In such microorganisms, the majority of small molecules are taken up by members of the OprD outer membrane protein family. Here we show that OprD channels require a carboxyl group in the substrate for efficient transport, and based on this we have renamed the family Occ, for outer membrane carboxylate channels. As expected from pairwise sequence identities that range from 35%–50%, the Occ proteins share a similar architecture, with a slightly off-center constriction formed by the inward-folded extracellular loops L3 and L7 and residues in the barrel wall. The transport data demonstrate that Occ channels have a pronounced preference for substrates with a carboxyl group, due to the universal presence of a basic ladder on one side of the barrel wall.

In addition to these new structures, we obtained much higher resolution data and more complete structures for OccD1 (formerly OprD; 2.15 Å versus 2.9 Å previously) and OccK1 (formerly OpdK; 1.65 Å versus 2.8 Å previously). As a comparison, the OccK1 pore is slightly larger in diameter than that of E. coli LamB, which is a channel specific for sugars. For OccK channels, conductance values are on average somewhat larger than those of OccD subfamily members, ranging from ∼50 pS for OccK4 to ∼300 pS for OccK1, OccK5, and OccK7. Vanillate, while being transported by OccK1, is clearly not the preferred substrate for this channel since relatively high substrate concentrations (10 µM) and long uptake times had to be used to obtain relatively low specific activities. This result is consistent with previous single-channel experiments, where the affinity of vanillate for OccK1 was found to be quite low (∼2 mM). Notably, while the current OccK1 structure contains two vanillate molecules, they are not bound at positions relevant for transport, confirming that vanillate is not a good substrate for OccK1. An interesting finding is the efficient lowering of OccK1-mediated benzoate transport by octanoate and caproate, suggesting that OccK1, but not OccD1 and OccK2, can serve as an uptake channel for medium-chain and possibly short-chain fatty acids. OccK1 is the least specific channel, also allowing the efficient passage of certain linear compounds such as medium-chain fatty acids. As judged by the inhibition of transport, OccK1 interacts with carbenicillin and cefoxitin. Intriguingly, OccK1-mediated transport is also affected by tetracycline, which is a non-β-lactam polyketide compound that does not have a carboxyl group.

>[2x]AEGGFLEDAKTDLVLRNYYFNRDFRDHDAGKSLVDEWAQGFILKFSSGYTPGTVGVGLDAIGLFGVKLNSGRGTSNSELLPLHDDGRAADNYGRVGVAAKLRVSASELKIGEMLPDIPLLRYDDGRLLPQTFRGFAVVSRELPGLALQAGRFDAVSLRNSADMQDLSAWSAPTQKSDGFNYAGAEYRFNRERTQLGLWHGQLEDVYRQSYANLLHKQRVGDWTLGANLGLFVDRDDGAARAGEIDSHTVYGLFSAGIGLHTFYLGLQKVGGDSGWQSVYGSSGRSMGNDMFNGNFTNADERSWQVRYDYDFVGLGWPGLIGMVRYGHGSNATTKAGSGGKEWERDVELGYTVQSGPLARLNVRLNHASNRRSFNSDFDQTRLVVSYPLSWGGHHHHHH> MRALVSFALFCVLYISVQGKVSSPKIQVYSHYPGEYGKENTLICYVSGFH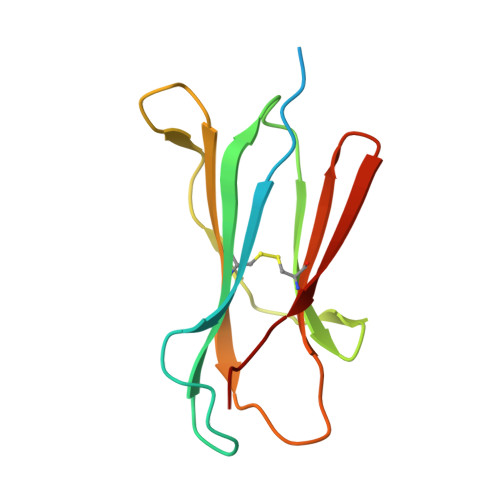PPDISIELLKNGEVIADAQQTDLAFEKGWQFHLTKSVSFKPEKSDEYSCSVRHMSKTKKIVWESNM>[2x]AASSAQCDFGGPFQAYKSVNGPGNGGYYLRKTTKPGTPECAYVLVPQNTLSEGQSTSFTYGKLQNGQMIQLTATVTVNGDKIEVTGAGQDLSGTTTVLFSDYRSCD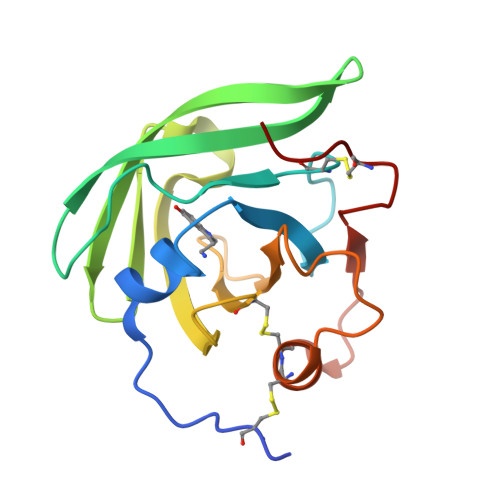VMRGPDGNYELWVHSSAINLQSYGCCDTKFAQVAGGRPIHHTWQTYCPPLP> GSAASLPKRIIKETEKLVSDPVPGITAEPHDDNLRYFQVTIEGPEQSPYEDGIFELELYLPDDYPMEAPKVRFLTKIYHPNIDRLGRICLDVLKTNWSPALQIRTVLLSIQALLASPNPNDPLANDVAEDWIKNEQGAKAKAREWTKLYAKKKPE;> HMSKVPRNFRLLEELEKGEKGFGPESCSYGLADSDDITMTKWNGTIL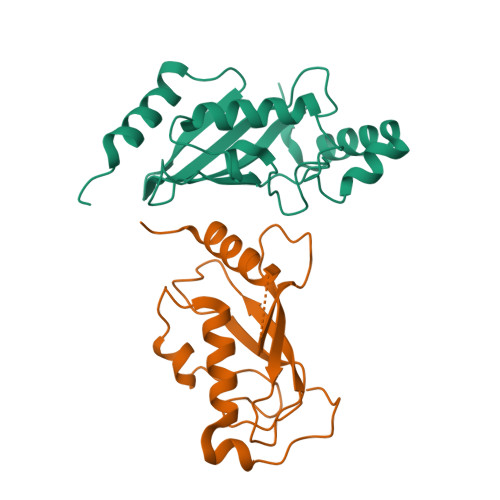GPPHSNHENRIYSLSIDCGPNYPDSPPKVTFISKINLPCVNPTTGEVQTDFHTLRDWKRAYTMETLLLDLRKEMATPANKKLRQPKEGETF>MHHHHHHYQLKIEGQAPGTCGSDKSLLVSALANGIGLPYECASGGCGVCKFELLEGTVQSMWPDAPGLSSRDREKGNRHLACQCIALSDLRIKVAVQDKYIPAIPISKMEAEVVAVRALTHDLLSVKLRTDVPANFLPGQFCLIEAEQLPGVVRAYSMANSMNPDGFWEFYIKRVPTGRFSPWLFENRKVGARLFLTGPMGTSFFRPGTGRKSLCIGGGAGLSYAAAIARASIRETDKPVKLFYGSRTPRDAVRWIDIDIDEDKLEVVQAVTEDTDS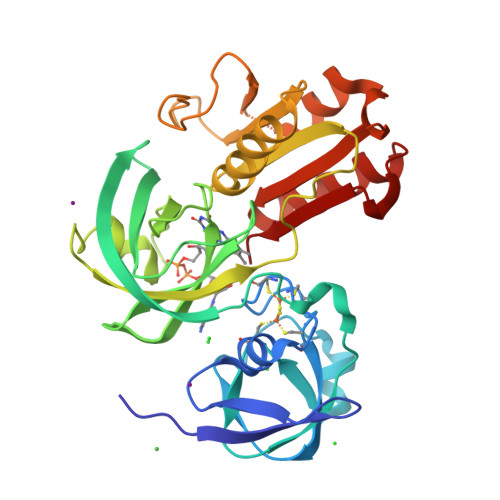LWQGPIGFIHQVVDAALLETLPEYEIYLAGPPPMVDATVRMLLGKGVPRDQIHFDAFF[3x]>[24x]MTLKVILGEHQITRTELLVGIATVSGCGAVVYCISKFWGYGAIAPYPQSGGNRVTRALQRAVIDKTKTPIET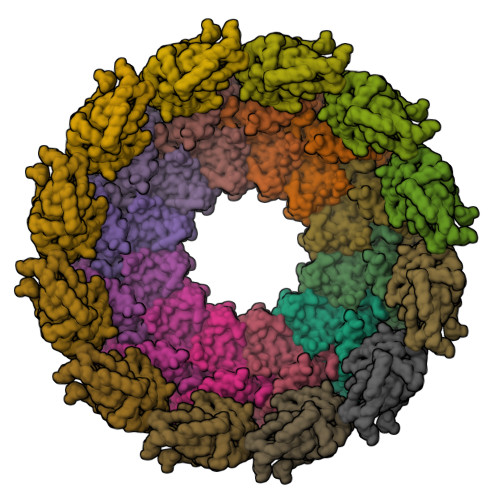RFYPLDSLRTVTPKRVADNGHAVSGAVRDAARRLIDESITAVGGSKFEVNPNPNSSTGLRNHFHFAVGDLAQDFRNDTPADDAFIVGVDVDYYVTEPDVLLEHMRPVVLHTFNPKKVSGFDADSPFTIKNNLVEYKVSGGAAWVHPVWDWCEAGEFIASRVRTSWKEWFLQLPLRMIGLEKVGYHKIHHCRPWTDCPDRALVYTIPQYVIWRFNWIDTELHVRKLKRIEYQDETKPGWNRLEYVTDKNELLVSIGREGEHAQITIEKEKLDMLSGLSATQSVNARLIGMGHKDPQYTSMIVQYYTGKKVVSPISPTVYKPTMPRVHWPVTSDADVPEVSARQYTLPIVSDCMMMPMIKRWETMSESIERRVTFVANDKKPSDRIAKIAETFVKLMNGPFKDLDPLSIEETIERLNKPSQQLQLRAVFEMIGVKPRQLIESFNKNEPGMKSSRIISGFPDILFILKVSRYTLAYSDIVLHAEHNEHWYYPGRNPTEIADGVCEFVSDCDAEVIETDFSNLDGRVSSWMQRNIAQKAMVQAFRPEYRDEIISFMDTIINCPAKAKRFGFRYEPGVGVKSGSPTTTPHNTQYNGCVEFTALTFEHPDAEPEDLFRLIGPKCGDDGLSRAIIQKSINRAAKCFGLELKVERYNPEIGLCFLSRVFVDPLATTTTIQDPLRTLRKLHLTTRDPTIPLADAACDRVEGYLCTDALTPLISDYCKMVLRLYGPTASTEQVRNQRRSRNKEKPYWLTCDGSWPQHPQDAHLMKQVLIKRTAIDEDQVDALIGRFAAMKDVWEKITHDSEESAAACTFDEDGVAPNSVDESLPLLNDAKQTRANPGTSRPHSNGGGSSHGNELPRRTEQRAQGPRQPARLPKQGKTNGKSDGNITAGETQRGGIPRGKGPRGGKTNTRRTPPKAGAQPQPSNNRKSRLEEELRRRLTE>[2x]MAITSNEIGTHDGYDYEFWKDSGGSGSMTLNSGGTFSAQWSNVNNILFRKGKKFDETQTHQQIGNMSINYGATYNPNGNSYLTVYGWTVDPLVEFYIVDSWGTWRPPGGTPKGTIN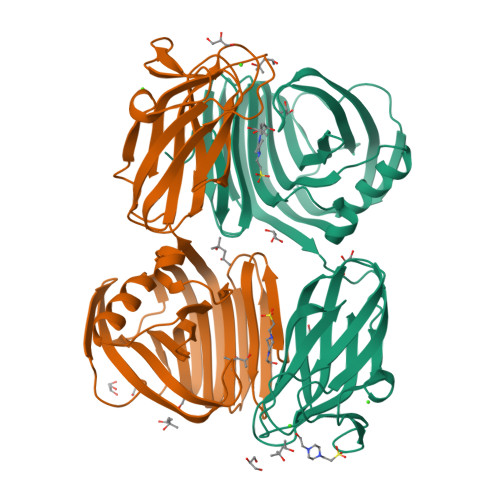VDGGTYQIYETTRYNQPSIKGTATFQQYWSVRTSKRTSGTISVSEHFRAWESLGMNMGNMYEVALTVEGYQSSGSANVYSNTLTIGGQSGGEQATRVEAESMTKGGPYTSNITSPFNGVALYANGDNVSFNHSFTKANSSFSLRGASNNSNMARVDLRIGGQNRGTFYFGDQYPAVYTINNINHGIGNQLVELIVTADDGTWDAYLDYLEIR>MSKTQAFRPLTLPPKLSLSDFNEFIQDIIRIVGSENVEVISSKDQIVDGSYMKPTHTHDPHHVMDQDYFLASAIVAPRNVADVQSIVGLANKFSFPLWPISIGRNSGYGGAAPRVSGSVVLDMGKNMNRVLEVNVEGAYCVVEPGVTYHDLHNYLEANNLRDKLWLDVPSLGGGSVLGNAVERGVGYTPYGDHWMMHSGMEVVLANGELLRTGMGALPDPKRPETMGLKPEDQPWSKIAHLFPYGFGPYIDGLFSQSNMGIVTKIGIWLMPNPGGYQSYLITLPKDGDLKQAVDIIRPLRLGMALQNVPTIRHILLDAAVLGDKRSYSSRTEPLSDEELDKIAKQLNLGRWNFYGALYGPEPI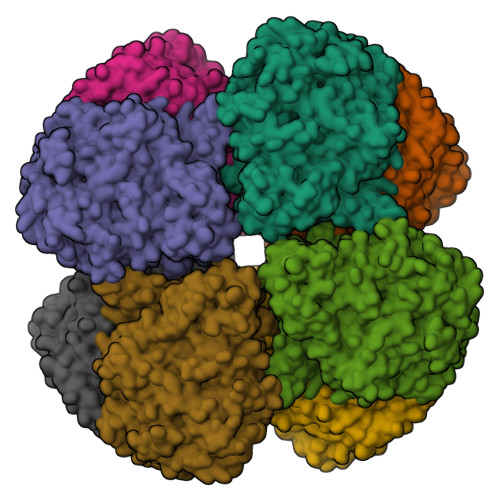RRVLWETIKDAFSAIPGVKFYFPEDTPENSVLRVRDKTMQGIPTYDELKWIDWLPNGAHLFFSPIAKVSGEDAMMQYAVTKKRCQEAGLDFIGTFTVGMREMHHIVCIVFNKKDLIQKRKVQWLMRTLIDDCAANGWGEYRTHLAFMDQIMETYNWNNSSFLRFNEVLKNAVDPNGIIAPGKSGVWPSQYSHVTWKL[2x]4-BROMOPHENOL 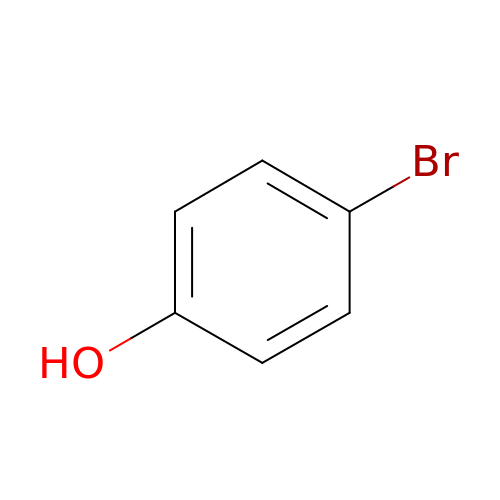| C6 H5 Br O | GZFGOTFRPZRKDS-UHFFFAOYSA-N> MNLEMLESQPVPEIDTLREEIDRLDAEILALVKRRAEVSKAIGKARMASGGPRLVHSREMKVI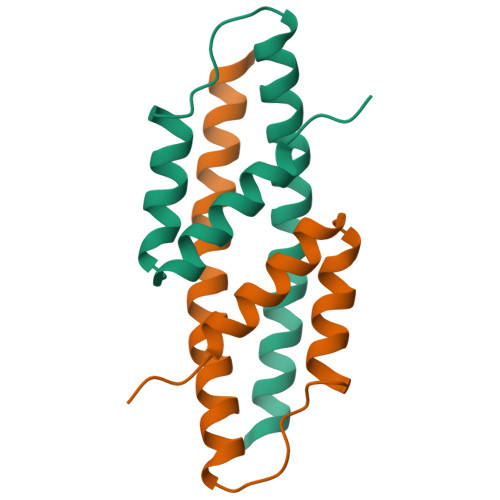ERYSELGPDGKDLAILLLRLGRGRLGH5-cyclopropyl-N-[1-(methylsulfonyl)piperidin-4-yl]-1,2-oxazole-3-carboxamide | C13 H19 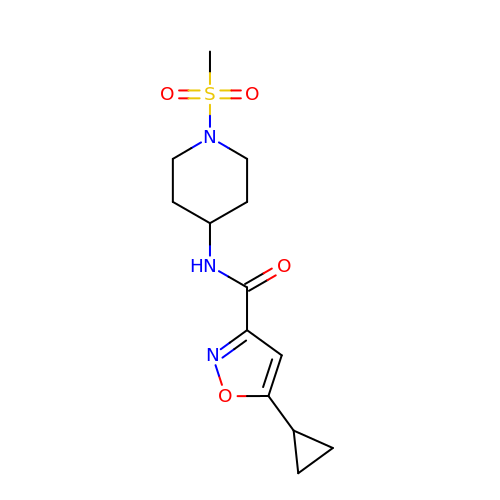N3 O4 S | KHFWLXQEZOVIGK-UHFFFAOYSA-N>[2x]SNAANNLGSKLLVGYWHNFDNGTGIIKLRDVSPKWDVINVSFGETGGDRSTVEFSPVYGTDAEFKSDISYLKSKGKKVVLSIGGQNGVVLLPDNAAKQRFINSIQSLIDK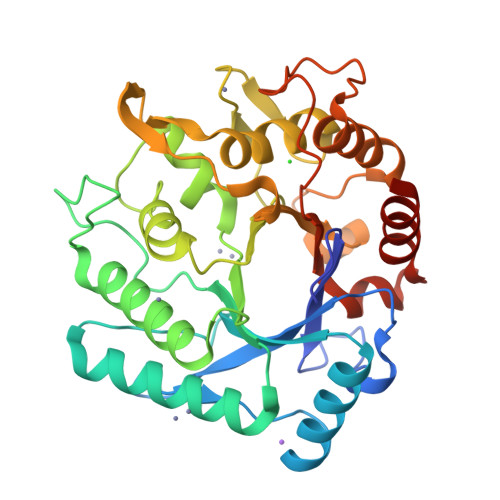YGFDGIDIDLESGIYLNGNDTNFKNPTTPQIVNLISAIRTISDHYGPDFLLSMAPETAYVQGGYSAYRSIWGAYLPIIYGVKDKLTYIHVQHYNAGSGIGMDGNNYNQGTADYEVAMADMLLHGFPIGGNANNMFPALRSDQVMIGLPATPAAAPSGGYISPTEMKKALDYIIKGIPFGGKYKLSNESGYPAFRGLMSWSINWDAKNNFEFSSNYRTYFDAIPLQK> NECLGTIGPVTPLDASDFALDIRMPGVTPKESDTYFCMSMRLPVDEEAFVIDFKPRASMDTVHHMLLFGCNMPSSTGSYWFCDEGTCTDK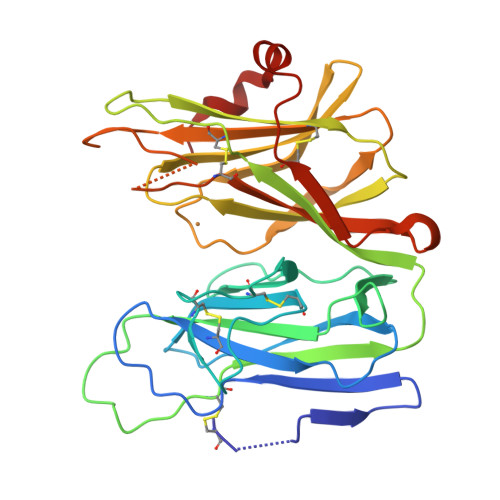ANILYAWARNAPPTRLPKGVGFRVGGETGSKYFVLQVAYGDISAFRDNHKDCSGVSVHLTRVPQPLIAGMYLMMSVDTVIPPGEKVVNADISCQYKMYPMHVFAYRVHTHHLGKVVSGYRVRNGQWTLIGRQNPQLPQAFYPVEHPVDVTFGDILAARCVFTGEGRTEATHIGGTSSDEMCNLYIMYYMEAKYALSFMTCTKNVAPDMFRTIPAEANIPIPV> XW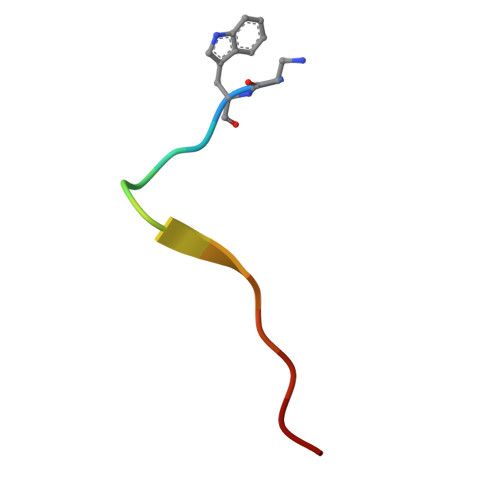LAYPDSVPYRPK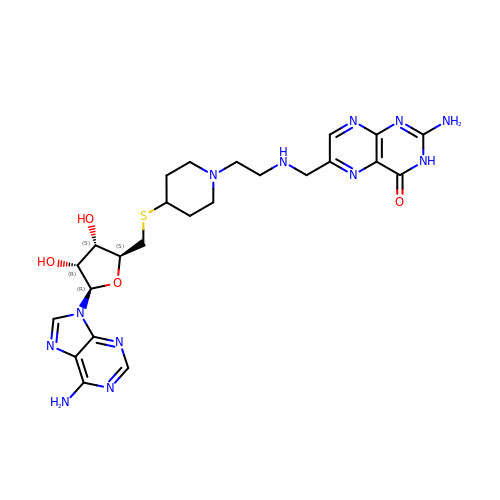5'-S-[1-(2-{[(2-amino-4-oxo-3,4-dihydropteridin-6-yl)methyl]amino}ethyl)piperidin-4-yl]-5'-thioadenosine | C24 H32 N12 O4 S | KWIHONXLDHOYOZ-YMYXXHFHSA-N>FDRNVPRICGVCGDRATGFHFNAMTCEGCKGF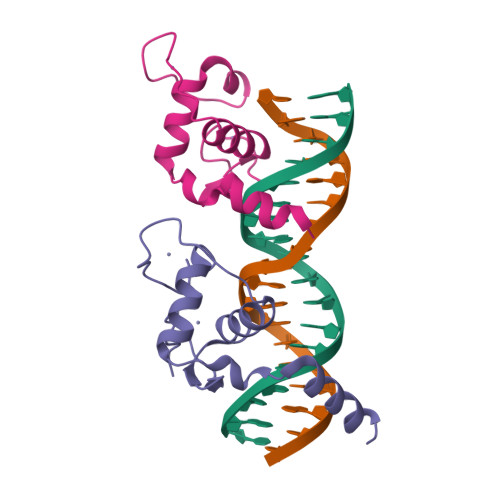FRRSMKRKALFTCPFNGDCRITKDNRRHCQACRLKRCVDIGMMKEFILTDEEVQRKREMILKRKEEEALKDSLRPKLS[2x]1-{5-[2-(morpholin-4-yl)ethoxy]-6-(pyridin-3-yl)[1,3]thiazolo[5,4-b]pyridin-2-yl}-3-prop-2-en-1-ylurea 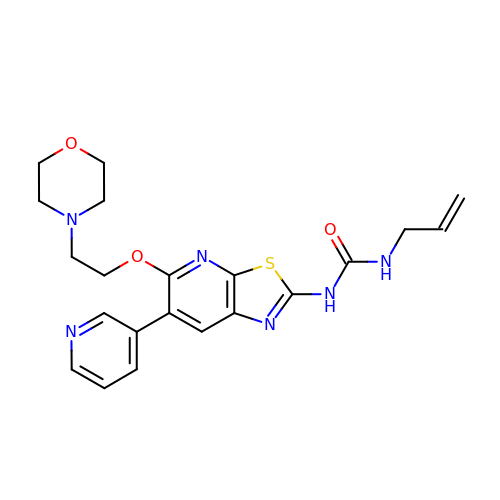| C21 H24 N6 O3 S | AQPJGKCFASTZAW-UHFFFAOYSA-N>[8x]AKTE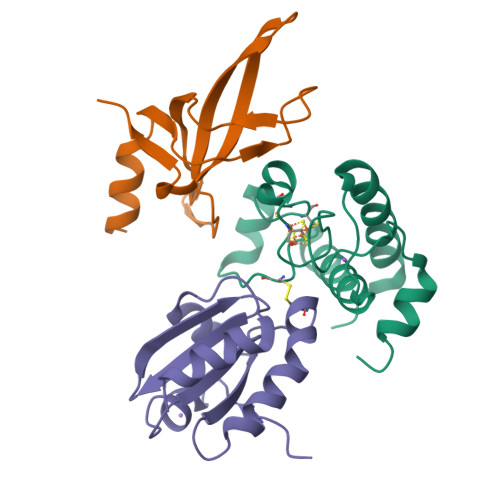PSEKSVEIMRKFSEQYARRSGTYFCVDKGVTSVVIKGLAEHKDSYGAPLCPCRHYDDKAAEVGQGFWNCPCVPMRERKECHCMLFLTPDNDFAGKDQTITSDEIKETTANM;>[7x]DIAVKSAASVDADADLSSSTSLETEEDEKAKEKIGARVRVTVPLKVYHVVRVPEVELMGMEGFIKDYVVLWKGKKISANLPFKVQFVKEIEGRGPVKFFTHLKEDEFELIDP;>CEAQETTTDIQVVNDSTWDSLVLKATGPVVVDFWAPWCGPSKMIDPLVNDLAQHYTGKIKFYKLNTDESPNTPGQYGVRSIPTIMIFVGGEKKDTIIGAVPKTTLTSSLDKFLP[8x]> IEAKKQTFDSFEDLLVNSDKPVLVDYYATWCGPSQFMVPILNEVSETLKDKIQVVKIDT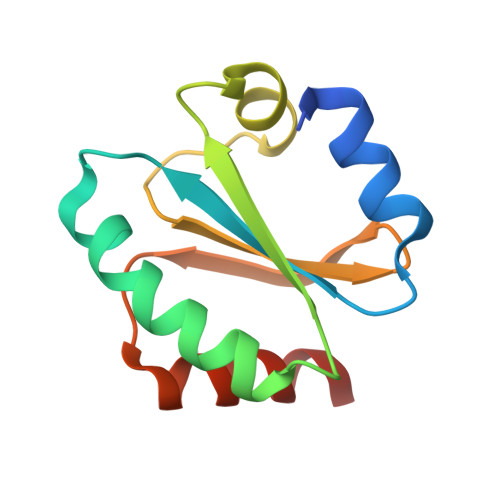EKYPSIANKYKIEALPTFILFKDGEPCDRFEGALTAKQLIQRIEDSLKVKP> MLSPKAATLAERSAGLAFSLYQAMAKDQAVENILLSPVVVASSLGLVSLGGKATTASQAKAVLSAEQLRDEEVHAGLGELLRSLSNSTARNVTWKLGSRLYGPSSVSFAEDFVRSSKQHYNCEHSKINFRDKRSALQSINEWAAQTTDGKLPEVTKDVERTDGALLVNAMFFKPHWDEKFHHKMVDNRGFMVTRSYTVGVTMMHRTGLYNYYDDEKEKLQIV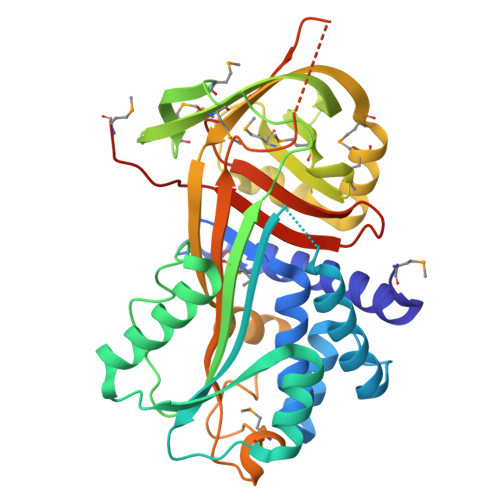EMPLAHKLSSLIILMPHHVEPLERLEKLLTKEQLKIWMGKMQKKAVAISLPKGVVEVTHDLQKHLAGLGLTEAIDKNKSDLSRMSGKKDLYLASVFHATAFEWDTEGNPFDQDIYGREELRSPKLFYADHPFIFLVRDTQSGSLLFIGRLVRPKGDKMRDELLEHHHHHH1,1,1-TRIFLUORO-3-(OCTYLTHIO)ACETONE | 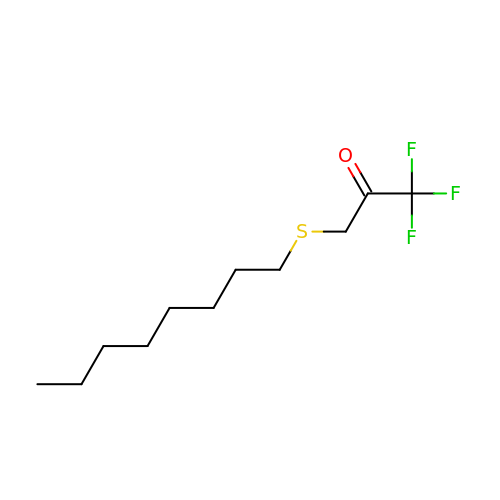C11 H19 F3 O S | WMQHRXUKAYSPPK-UHFFFAOYSA-N>MVMNNEYFKLYTDSQFLSPYAFTVFVGLHEKQIPFEIAAIDLGQQGQFETSFVEKSLTAKVPVLEHNDFALSESSAILEYLEELYPDTAIYPKDIQARARARQIQAWLRSDLVALRTERPTDVIFIQPKSTPLSEEGKKAAEKLFFVAEKLLASDAEFLFGSWSIVDAELALMLQRLI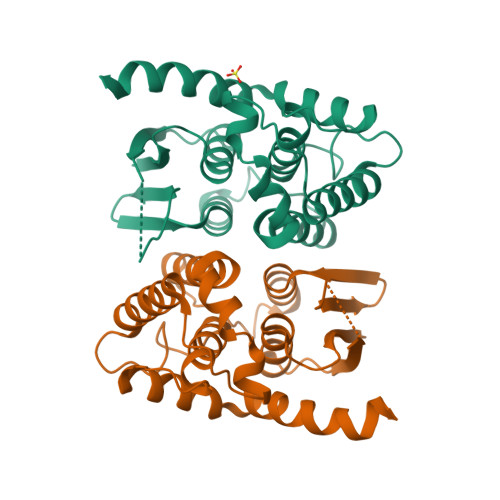QNGDAVSERLKNYALQQWQRPSVQKWLALRHKAENLYFQ[3x]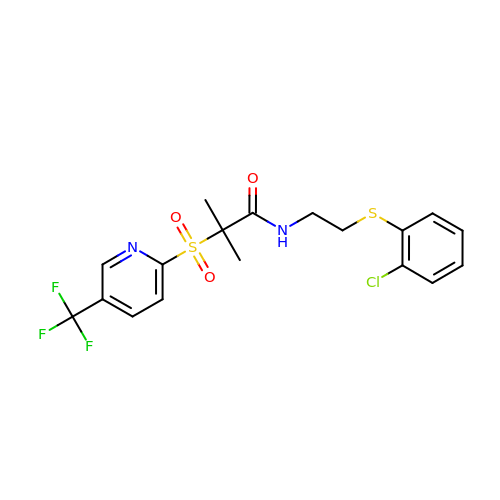N-{2-[(2-chlorophenyl)sulfanyl]ethyl}-2-methyl-2-{[5-(trifluoromethyl)pyridin-2-yl]sulfonyl}propanamide | C18 H18 Cl F3 N2 O3 S2 | OUZIIFOEMPAZKX-UHFFFAOYSA-N Transforming growth factor-β receptor type 3 (TGFR-3), also known as betaglycan, is an ubiquitously expressed cell surface proteoglycan that serves as a co-receptor for members of the TGF-β family of cystein knot growth factors, i.e. TGF-βs, activins, inhibins, growth differentiation factors (GDFs) and the bone morphogenetic proteins (BMPs). Many TGF-β family members bind to TGFR-3 first, and this interaction subsequently facilitates the formation of a ternary signaling complex between the growth factor and the receptors TGFR-1 and TGFR-2. The 785 residue-long ectodomain of TGFR-3 can be subdivided into two halves of similar lengths. The C-terminal half contains next to a bioinformatically delineated ZP core domain (residues 454 to 728) a so-called external hydrophobic patch (EHP) that is part of a stretch of amino acids that connects the ZP domain to the membrane-spanning segment in TGFR-3.

The mouse TGFR-3-ZP protein was crystallized in the presence of the endoglycosidase F3 under the assumption that in situ deglycosylation facilitates crystallization. Surprisingly, the structure determination revealed that the crystals did not contain the entire TGFR-3-ZP domain but only a fragment that corresponds to the ZP-C subdomain. The polypeptide chain could be traced contiguously from residues 591 to 757 with the exception of a stretch of 11 residues that is part of the FG loop (residues 730 to 744). In case of the bridging residues 730 to 744 in the FG loop we observe residual, however non-interpretable, difference density hinting that this segment remained largely intact in the crystals and that the lack of defined electron density is caused by conformational disorder in this segment. As previously seen in rat TGFR-3 and other ZP domain containing proteins, the overall fold topology is reminiscent of the immunoglobulin superfold and comprises a β-sheet sandwich formed by two four-stranded β-sheets (strands A, B, E, D and C’, C, F, G). The intervening loop segments (termed AB, BC, CC’, …) differ considerably in size and in case of loop FG also contains a small α-helical segment termed αFG.With the exception of strand G (residues 745 to 757 in murine TGFR-3, see below) the structure compares well to the corresponding rat ZP-C fragment, which was used as a search model during molecular replacement. Overall, the root mean square (r.m.s.) deviation between common main chain atoms in the rat and mouse structure is 0.7 Å. Unexpectedly, the amino acid registration of strand G is shifted by four residues in murine ZP-C when compared to the corresponding segment in rat ZP-C. We therefore conclude that the shift in the registration of strand G, which contains the EHP sequence, constitutes a genuine difference between both structures.

> TFNMELYNTDLFLVPSPGVFSVAENEHVYVEVSVTKADQDLGFAIQTCFISPYSNPDRMSDYTIIENICPKDDSVKFYSSKRVHFPIPHAEVDKKRFSFVFKSVFNTSLLFLHCELTLCSRNKGSQKLPKCVTPDDACTSLDATMIWTMMQNKKTFTKPLAVVLQVD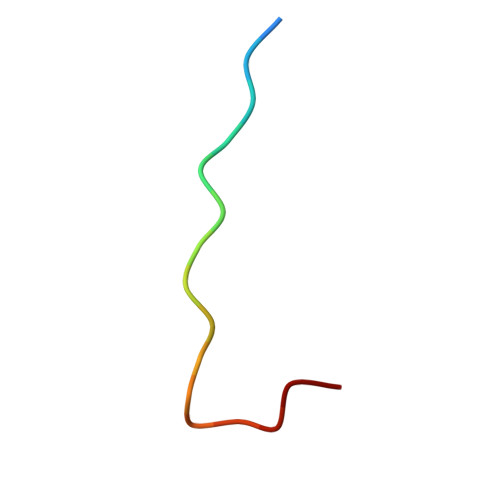> KAFVHMPTLPNLDFHKT> MSAAPVLSITNASVVYPDGISTVTALDSANVEIFPGELVAIVGESGSGKSTLLSIAGFLQEPTSGTVTLHGAEGLDATSTRREHIGFVFQQPNLLGSLTAREQLLITDHLRGIKPRKDRADELLARVGLKGLGGRRVAQLSGGQRQRVNIARALMGNPQLLLADEPTSALDARLSKEIVELLRDVTKEFALATLMVTHDRSQLAYADRFVEMADGKALQTA;> MFLGIRDIRAAAGRFALIASVVGLITLLI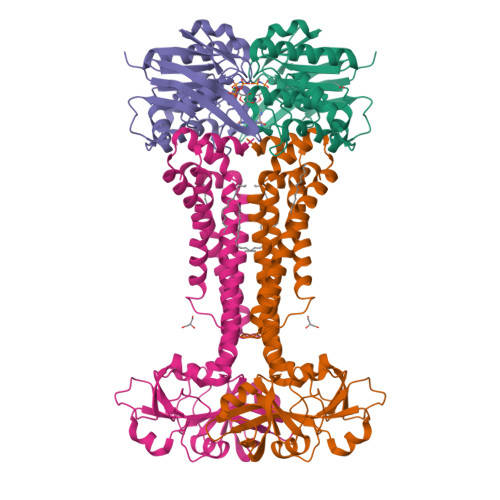VMLTGLTQGLGKQNTSAIEALAPHSVVFTTAGGSSPEFTSSEISEQQAERWKDSTPLGVSQTRIESDQNANTTAVMGLPEGTPLPDSVGGFIEQGALLPAELADFLHVRAGDHITLGGATVTVAGTVKTENYSHTPVVWVDTATWQLVSHTKAVGTVLLLNQEPTIQPQDNEVVTDLKGAFQAMPAYKSERSSLLSMQAFLYIISALVTVAFLTVWTLQRTRDIAVLAALGASKRYLLIDALGQAAIILAAGVALGAGIGALLGWLIAGSVPFSLGWVSVLGPALGIWLLGLIGATIAVRNVTKVDPQIALGATA> GAMDPEFMDGTAAEPRPGAGSLQHAQPPPQPRKKRPEDFKFGKILGEGSFSTVVLARELATSREYAIKILEKRHIIKENKVPYVTRERDVMSRLDHPFFVKLYFCFQDDEKLYFGLSYAKNGELLKYIRKIGSFDETCTRFYTAEIVSALEYLHGKGIIHRDLKPENILLNEDMHIQITDFGTAKVLSPESKQARANSFVGTAQYVSPELLTEKSACKSSDLWALGCIIY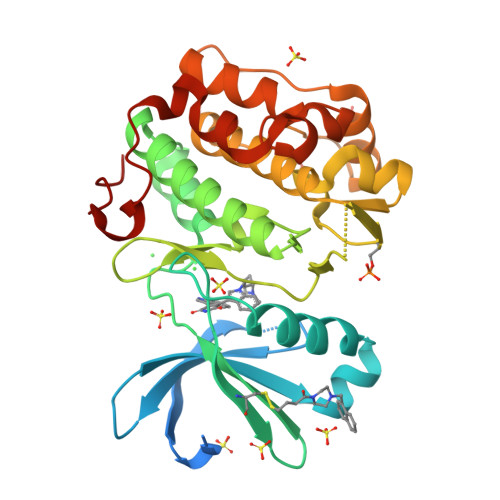QLVAGLPPFRAGNEYLIFQKIIKLEYDFPEKFFPKARDLVEKLLVLDATKRLGCEEMEGYGPLKAHPFFESVTWENLHQQTPPKLT> PRQIPFIIGNEACERFSFYGMRNILVQFLITSLLLQEVGAPERDAEAKHILHSFMIGVFFFPLLGGWLADRFFGKYTTIIWFSLIYCAGHACLALFEDSRSGFFVGLGLIAFGAGGIKPLVASFMVDQFDQSNKHRAKVVFDAFYWIINFGSLFASLLIPLALKHLGPSWAFGIPGILMFIATAVFWLGRKRYVRVPLPPKDPHGFGAVVRSALLAHAPGQ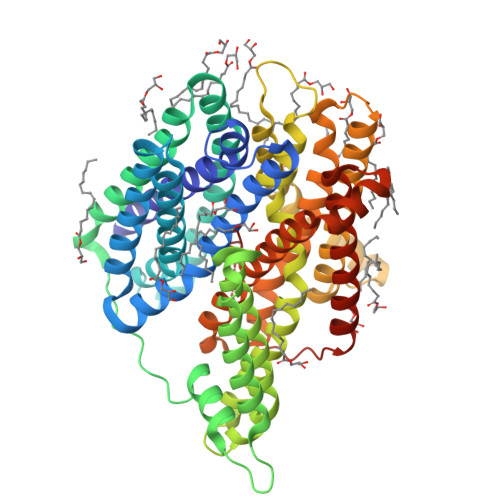GRPGLALAAISVLLALACLGLTEQLGLVICLCMALVLLLAGIGGGTWWQLERARGTHPDAAVDGVRALLRVLVIFALVTPFFSLFDQKASTWVLQGREMRMPAWFTASQMQALNPLLVMLLIPFNNLVLYPLLRRLGWEPTSLRRMTSGIAFSGVAWIAVGAIQVAMDGGEPMHIAWQILPYALLTFGEVLVSATGIEFAYSQAPPSMKGVVMSFWYLTTTVGNLWVLLSNVAVRNATVTSHIADTGLSEAAFLMFFFAAFAFLAALAFGLYARRYRMVDNYRPAGSENLYFQ>[4x]MLAKNKGKIPGLKIDQKIRGQMPERGWTEDDIKNTVSNGATGT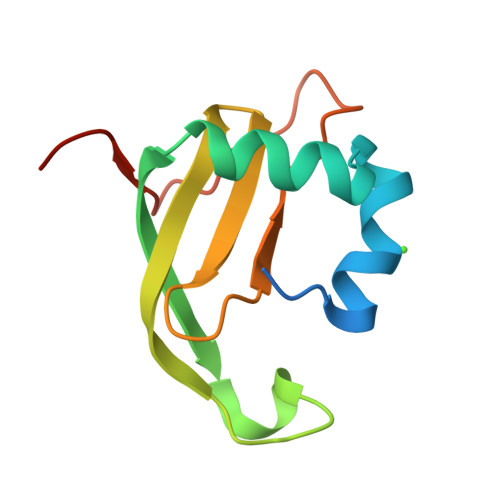SFDKRSPKKTPPDYLGRNDPATVYGSPGKYVVVNDRTGEVTQISDKTDPGWVDDSRIQWGNKNDQ Cytoplasmic dynein-1 (dynein) is the main minus-end-directed microtubule motor responsible for transporting vesicles, protein complexes, RNAs, organelles, and viruses along microtubules. Dynein is autoinhibited and undergoes conformational changes to form an active complex that consists of one or two dynein dimers, the dynactin complex, and activating adapter(s). Dynein function in vivo also requires Lis1, which is an essential positive regulator of dynein, as shown by genetic studies in many organisms. Lis1 is required for active dynein complexes to form, but how it enables this is unclear.

Here, we present a structure of two yeast dynein motor domains with two Lis1 dimers wedged in-between. Importantly, the Chi conformation is not a consequence of the E2488Q substitution in dynein, or the use of ATP-vanadate in the sample: we also observed Chi in a data set collected from a sample containing wild-type dynein monomer, ATP, and Lis1. The AAA5 and AAA6 Chi-specific interactions involve residues on Lis1’s β-propeller that are different from those involved in all previously characterized Lis1–dynein and Lis1–Lis1 contacts. To disrupt the Chi-specific interactions, we mutated Asn213 in Lis1 to Ala (Lis1N213A), Trp288 to Asp (Lis1W288D), or both (Lis1N213A W288D) in the endogenous locus of yeast Lis1 (PAC1; GeneID: 854443). On the basis of our structure, we introduced F3446A in AAA5 and E3867A in AAA6 (Dyn1F3446A E3867A). Although we did not build the side chain for E3867 in our model owing to the lower resolution of that part of the map, this residue is a good candidate for mediating the interaction between dynein and Lis1-N213.

> GDQLTHVVEEVKTYDLVWRSIKNLWEDVQRTFETPWCRVDVLLLQSDLANFLRRADELPRAVKQFEMYKSLFSQVNMLTSVNKILVELKDGALKPRHWNMIFRDIGKRQIQKNLLDKLEFSLKDVMVLNLTLNEILLTKIIERAQKEFVIEKSLNRIKKFWKEAQYEVIEHSSGLKLVREWDVLEQACKEDLEELVSMKASNYYKIFEQDCLDLESKLTKLSEIQVNWVEVQFYWLDLYGILGENLDIQNFLPLETSKFKSLTSEYKMITTRAFQLDTTIEVIHIPNFDTTLKLTIDSLKMIKSSLSTFLERQRRQFPRFYFLGNDDLLKIIGSGKHHDQVSKFMKKMFGSIESIIFFEDSITGVRSVEGEVLNLNEKIELKDSIQAQEWLNILDTEIKLSVFTQFRDCLGQLKDGTDIEVVVSKYIFQAILLSAQVMWTELVEKCLQTNEFSKYWKEVDMKIKGLLDKLNKSSDNVKKKIEALLVEYLHFNNVIGQLKNCSTKEEARLLWAKVQKFYQKNDTLDDLNSVFISQSGYLLQYKFEYIGIPERLIYTPLLLVGFATLTDSLHQKYGGCFFGPAGTGKTETVKAFGQNLGRVVVVFNCDDSFDYQVLSRLLVGITQIGAWGCFDEFNRLDEKVLSAVSANIQQIQNGLQVGKSHITLLEEETPLSPHTAVFITLNPGYNGRSELPENLKKSFREFSMKSPQSGTIAEMILQIMGFEDSKSLASKIVHFLELLSSKCSSMNHYHFGLRTLKGVLRNCSPLVSEFGEGEKTVVESLKRVILPSLGDTDELVFKDELSKIFDSAGTPLNSKAIVQCLKDAGQRSGFSMSEEFLKKCMQFYYMQKTQQALILVGKAGCGKTATWKTVIDAMAIFDGHANVVYVIDTKVLTKESLYGSMLKATLEWRDGLFTSILRRVNDDITGTFKNSRIWVVFDSDLDPEYVEAMNSVLDDNKILTLPNGERLPIPPNFRILFETDNLDHTTPATITRCGLLWFSTDVCSISSKIDHLLNKSYEALDNKLSMFELDKLKDLISDSFDMASLTNIFTCSNDLVHILGVRTFNKLETAVQLAVHLISSYRQWFQNLDDKSLKDVITLLIKRSLLYALAGDSTGESQRAFIQTINTYFGHDSQELSDYSTIVIANDKLSFSSFCSEIPSVSLEAHEVMRPDIVIPTIDTIKHEKIFYDLLNSKRGIILCGPPGSGKTMIMNNALRNSSLYDVVGINFSKDTTTEHILSALHRHTNYVTTSKGLTLLPKSDIKNLVLFCDQINLPKLDKYGSQNVVLFLRQLMEKQGFWKTPENKWVTIERIHIVGACNPPTDPGRIPMSERFTRHAAILYLGYPSGKSLSQIYEIYYKAIFKLVPEFRSYTEPFARASVHLYNECKARYSTGLQSHYLFSPRELTRLVRGVYTAINTGPRQTLRSLIRLWAYEAWRIFADRLVGVKEKNSFEQLLYETVDKYLPNQDLGNISSTSLLFSGLLSLDFKEVNKTDLVNFIEERFKTFCDEELEVPMVIHESMVDHILRIDRALKQVQGHMMLIGASRTGKTILTRFVAWLNGLKIVQPKIHRHSNLSDFDMILKKAISDCSLKESRTCLIIDESNILETAFLERMNTLLANADIPDLFQGEEYDKLLNNLRNKTRSLGLLLDTEQELYDWFVGEIAKNLHVVFTICDPTNNKSSAMISSPALFNRCIINWMGDWDTKTMSQVANNMVDVVPMEFTDFIVPEVNKELVFTEPIQTIRDAVVNILIHFDRNFYQKMKVGVNPRSPGYFIDGLRALVKLVTAKYQDLQENQRFVNVGLEKLNESVLKVNELNKTLSKKSTELTEKEKEARSTLDKMLMEQNESERKQEATEEIKKILKVQEEDIRKRKEVVMKSIQDIEPTILEAQRGVKNIKKQQLTEIRSMVNPPSGVKIVMEAVCAILGYQFSNWRDIQQFIRKDDFIHNIVHYDTTLHMKPQIRKYMEEEFLSDPNFTYETINRASKACGPLYQWVNAQINFSKVLENVDPLRQEMKRIEFESLKTKANLLAAEEMTQDLEASIEVSKQKYSLLIRDVEAIKTEMSNVQANLDRSISLVKSLTFEKERWLNTTKQFSKTSQELIGNCIISSIYETYFGHLNERERGDMLVILKRLLGKFAVKYDVNYRFIDYLVTLDEKMKWLECGLDKNDYFLENMSIVMNSQDAVPFLLDPSSHMITVISNYYGNKTVLLSFLEEGFVKRLENAVRFGSVVIIQDGEFFDPIISRLISREFNHAGNRVTVEIGDHEVDVSGDFKLFIHSCDPSGDIPIFLRSRVRLVHFVTNKESIETRIFDITLTEENAEMQRKREDLIKLNTEYRLKLKNLEKRLLEELNNSQGNMLENDELMVTLNNLKKEAMNIEKKLSESEEFFPQFDNLVEEYSIIGKHSVKIFSMLEKFGQFHWFYGISIGQFLSCFKRVFIKKSRETRAARTRVDEILWLLYQEVYCQFSTALDKKFKMIMAMTMFCLYKFDIESEQYKEAVLTMIGVLSESSDGVPKLTVDTNDDLRYLWDYVTTKSYISALNWFKNEFFVDEWNIADVVANSENNYFTMASERDVDGTFKLIELAKASKESLKIIPLGSIENLNYAQEEISKSKIEGGWILLQNIQMSLSWVKTYLHKHVEETKAAEEHEKFKMFMTCHLTGDKLPAPLLQRTDRVVYEDIPGILDTVKDLWGSQFFTGKISGVWSVYCTFLLSWFHALITARTRLVPHGFSKKYYFNDCDFQFASVYLENVLATNSTNNIPWAQVRDHIATIVYGGKIDEEKDLEVVAKLCAHVFCGSDNLQIVPGVRIPQPLLQQSEEEERARLTAILSNTIEPADSLSSWLQLPRESILDYERLQAKEVASSTEQLLQEM;>[2x]GMTNWQQQLPLTDTQKNELDKSVLRYLNWNYKQTVRHEHAQDYESVRHAIVTLSGFLLQESVDRQEFISNNDTSNESMVDIDELLLPKKWNSIVRLQKKIIELEQNTETLVSQIKDLNTQVSELAQFKPTTSNGTSAHNVLKWIPRNLPSCLINVESSVTSVKLHPNLPIVFVATDHGKLYAFDLFNYTIPLASLQSHTKAITSMDVLFTNYTNSSKKNYLVIVTASKDLQIHVFKWVSEECKFQQIRSLLGHEHIVSAVKIWQKNNDVHIASCSRDQTVKIWDFHNGWSLKTFQPHSQWVRSIDVLGDYIISGSHDTTLRLTHWPSGNGLSVGTGHEFPIEKVKFIHFIEDSPEIRFRTPSTDRYKNWGMQYCVSASRDRTIKIWEIPLPTLMAHRAPIPNPTDSNFRCVLTLKGHLSWVRDISIRGQYLFSCADDKSVRCWDLNTGQCLHVWEKLHTGFVNCLDLDVDFDSNVTPRQMMVTGGLDCKSNVFMR>[2x]MSMIKSYAAKEAGGELEVYEYDPGELRPQDVEVQVDYCGICHSDLSMIDNEWGFSQYPLVAGHEVIGRVVALGSAAQDKGLQVGQRVGIGWTARSCGHCDACISGNQINCEQGAVPTIMNRGGFAEKLRADWQWVIPLPENIDIESAGPLLCGGITVFKPLLMHHITATSRVGVIGIGGLGHIAIKLLHAMGCEVTAFSSNPAKEQEVLAMGADKVVNSRDPQALKALAGQFDLIINTVNVSLDWQPYFEALTYGGNFHTVGAVLTPLSVPAFTLIAGDRSVSGSATGTPYELRKLMRFAARSKVAPTTELFPMSKINDAIQHVRDGKARYRVVLKADYLAHHHHHH

Escherichia coli possess strong alcohol dehydrogenases that could contribute to producing alcohols through a designed pathway. These powerful enzymes, including YjgB, YahK, and YqhD, show nicotinamide adenine dinucleotide phosphate (NADP)-dependent activities for a variety of aldehydes. YqhD belongs to the family III metal-dependent polyol dehydrogenases, while YjgB and YahK are classified as members of the cinnamyl alcohol dehydrogenase family. As predicted from sequence alignment, the EcYjgB structure was found to belong to a typical cinnamyl alcohol dehydrogenase (CAD) family and sinapyl alcohol dehydrogenase (SAD) family, which consists of a nucleotide binding domain (NBD, residues 165–286) and a substrate-binding domain (SBD, residues 1–164 and 287–338). We observed a cleft between the SBD (substrate-binding domain) and NBD (nucleotide-binding domain) that forms the active site with a catalytic Zn2+ ion. It was found that the catalytic Zn2+ ion is coordinated by the tetrahedral combination of Cys41, His63, Glu64, and Cys152, which were well conserved.

The E. coli YjgB (EcYjgB) was crystallized in the monoclinic space group, C2, and its crystal structure was successfully determined at 1.55 Å resolution. The NBD (nucleotide-binding domain) was shown to adopt a canonical Rossmann fold that was composed of alternating beta strands and alpha helixes, which can hold cofactor NAD(H)/NADP(H). As in other Zn-dependent CAD and SAD families, PDBePISA (Proteins, Interfaces, Structures, and Assemblies) analysis showed that this Rossmann fold can form a dimer. The structure of the dimeric interface showed that dimerization region I (residues 268–270) and II (residues 280–284) establish the dimerization interface by generating two β-sheets. In the apo structure, distances ranging from 2.0 to 2.3 Å were shown between the zinc ion and its coordinated resides; Cys41 (2.3 Å), His63 (2.0 Å), Glu64 (2.0 Å), and Cys152 (2.3 Å).(1R,3R,4S)-4-[({6-[(4-CYANO-2-FLUOROBENZYL)OXY]NAPHTHALEN-2-YL}SULFONYL)AMINO]CYCLOHEXANE-1,3-DICARBOXYLIC 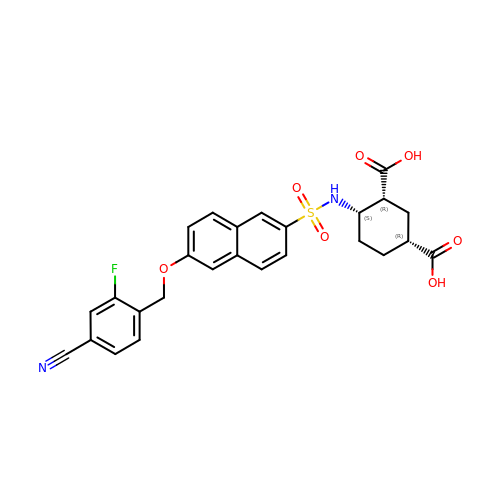ACID | C26 H23 F N2 O7 S | NYXJFBFDAFPUOG-XANCMCCPSA-N>[2x]MNLTEKGTKTAKLSASDRIIYADNHLIHGPDDITAYMKGVCYDAAAY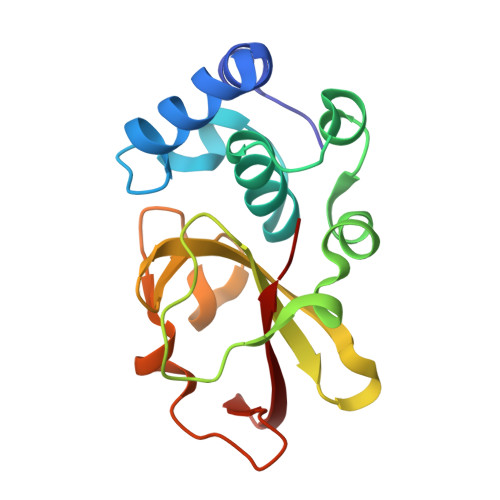MRYLYNAKISFDQLTSISAQNWLPVFKFAEGRMWDGRNSLPGGKAIGFCRVKGMEFFHAAVAVGGTEIRAINGGLLGAGWLHPVDLRKVLTQKNPDGSFKYDGTDIFVYISNL> MAVFRDLRHYIDTLTEKLGADEVQTIKGANWDLEIGCITELSAEKEGPALLFDDIPGYPSGHRVFTNFMGTVSRCAVALGLPADTSAMDIIRAWKDLGKRIEPIPPVEVSEGAILENVLEGDDVDLEMFPTPRWHDGDGGRYIGTACMVITRDPDTGWVNVGTYRGCVQGKDRLSLWMLGNRHALAIAKKYWDRGTACPIAVVVGCDPILTTAAAIAAPSGVCEYDVAGGLRGVGVEVISAPGTGLPIPANAEIVFEGEMPPVEEESVHEGPFGEWTGYFTHAGDETVVRVQRILHRDSPIILGAPPMIPTVPAGDQAVPLYSASVTWDHLEASGVQNIKGVWAYARQLMMVISIEQTGAGDAMHALLAAAGRKRTGGVDRYFVVVDEDIDITDINHVLWALFTRVDPAESIHVLRTPTTAIDPRLSPAKREAGDMSMGIVLIDACKPFAWKDSYPRANRFD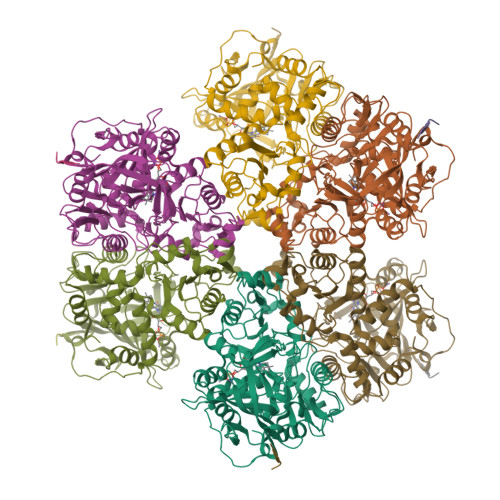EPYRAEIRDRWKATLPL>[2x]SKNSGNNSNNSSNNNSSNNTGGKKIKIGMVTDVGGVNDGSFNQSAWEGLQRAQKELGVEVRYAES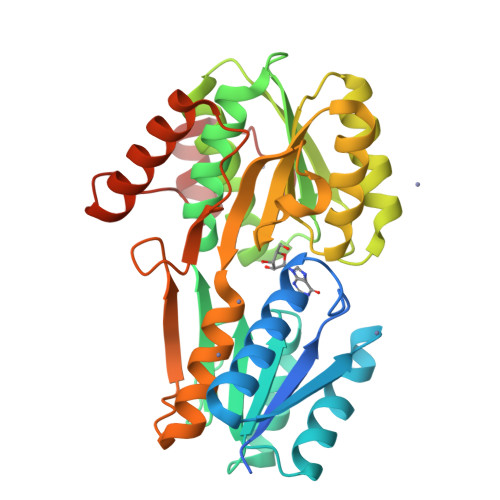ATDADYAPNIEAFIDEGYDLIICVGYMLADATRKAAEANPNQKFAIIDDASIDLPNVTCLMFEQSQASYLVGLVAGKMTKTNKVGFVVGMVSQTMNEFGYGYLAGVKDANPNATILQFNANSFSSTETGKSAATTMITNGADVIFHAAGGTGLGVIEGCKDAGKWAIGVDSDQSPLAPENILTSAMKRVDNACFDIAKAVKEGNVKPGIITYDLKSAGVDIAPTTTNLPKEVLDYVNQAKQDIINGKITVPKTKAEFEAKYGNIYELDD>SFELPALPYAKDALAPHISAETIEYHYGKHHQTYVTNLNNLIKGTAFEGKSLEEIIRSSEGGVFNNAAHVWNHTFYWNCLAPNAGGEPTGKVAEAIAASFGSFADFKAQFTDAAIKNFGSGWTWLVKNSDGKLAIVSTSNAGTPLTTDATPLLTV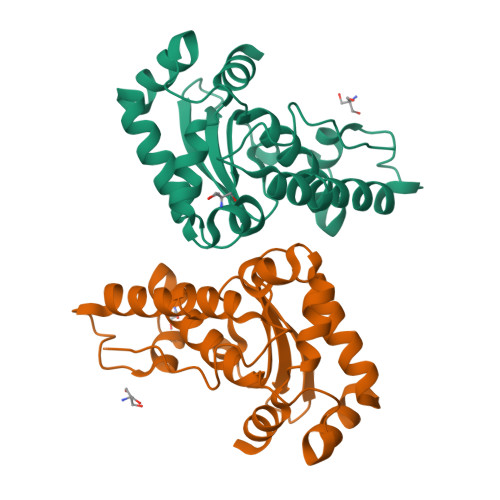DVWEHAYYIDYRNARPGYLEHFWALVNWEFVAKNLAA[2x]>SMEMNSVMHNDLKEVLLTEEDIQNICK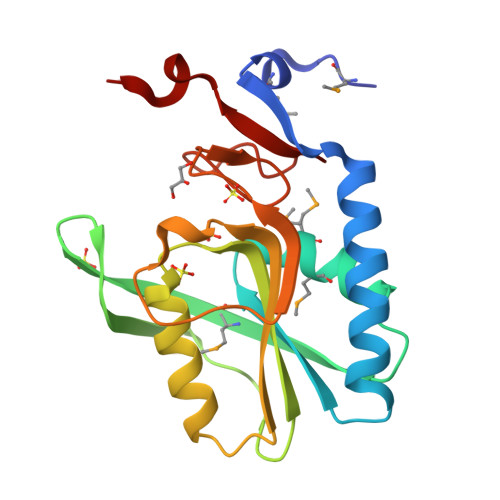ELGAQLTKDYQGKPLVCVGILKGSAMFMSDLIKRIDTHLSIDFMDVSSYHGGTESTGEVQIIKDLGSSIENKDVLIIEDILETGTTLKSITELLQSRKVNSLEIVTLLDKPNRRKADIEAKYVGKKIPDEFVVGYGLDYRELYRNLPYIGTLKPEVYSN[2x]>MADREHMFDKVVTPSDVGKLNRLVI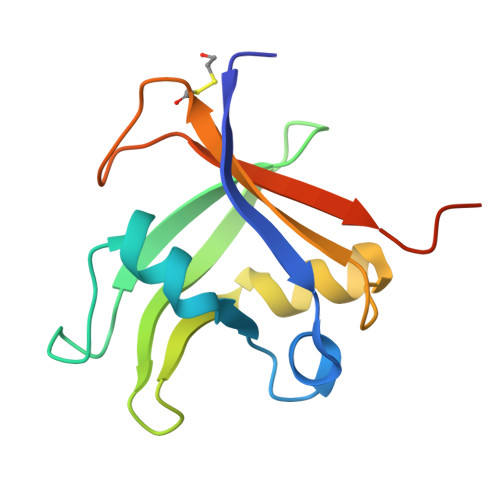PKQHAERFFPLDSSSNEKGLLLNFEDLTGKSWRFRYSYWNSSQSYVMTKGWSRFVKDKKLDAGDIVSFQRCVGDSGRDSRLFIDWRRRPKVGHHHHHHG[2x]>MRTRSTISTPNGITWYYEQEGTGPDVVLVPDGLGECQMFDSSVSQIAAQGFRVTTFDMPGMSRSAKAPPETYTEVTAQKLASYVISVLDALDIKHATVWGCASGASTVVALLLGYPDRIRNAMCHELPTKLLDHLSNTAVLEDEEISKILANVMLNDVSGGSEAWQAMGDEVHARLHKNYPVWARGYPRTIPPSAPVKDLEA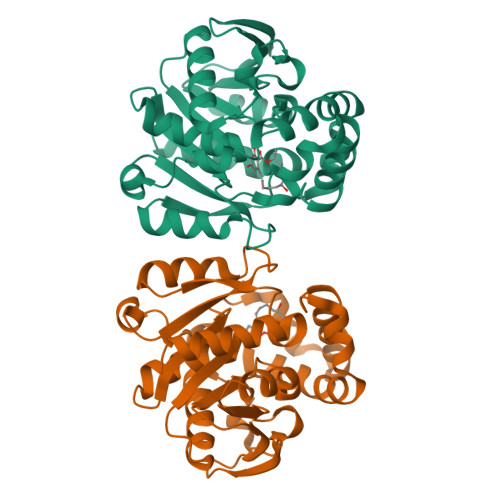LRGKPLDWTVGAATPTESFFDNIVTATKAGVNIGLLPGMHFPYVSHPDVFAKYVVETTQKHL[3x]>QLSPDIYAKSCPNLVQIVRKQVAIALKAEIRMAASLIRLHFHDCF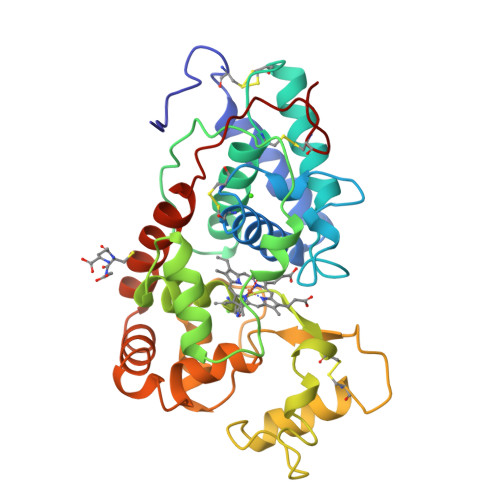VNGCDASLLLDGADSEKLAIPNINSARGFEVIDTIKAAVENACPGVVSCADILTLAARDSVVLSGGPGWRVALGRKDGLVANQNSANNLPSPFEPLDAIIAKFVAVNLNITDVVALSGAHTFGQAKCAVFSNRLFNFTGAGNPDATLETSLLSNLQTVCPLGGNSNITAPLDRSTTDTFDNNYFKNLLEGKGLLSSDQILFSSDLAVNTTKKLVEAYSRSQSLFFRDFTCAMIRMGNISNGASGEVRTNCRVINN[2x]> GSPGISGGGGGSAYSNTYQEFTNIDQAKAWGNAQYKKYGLSKSEKEAIVSYTKSASEINGKLRQNKGVINGFPSNLIKQVELLDKSFNKMKTPENIMLFRGDDPAYLGTEFQNTLLNSNGTINKTAFEKAKAKFLNKDRLEYGYISTSLMNVSQFAGRPIITKFKVAKGSKAG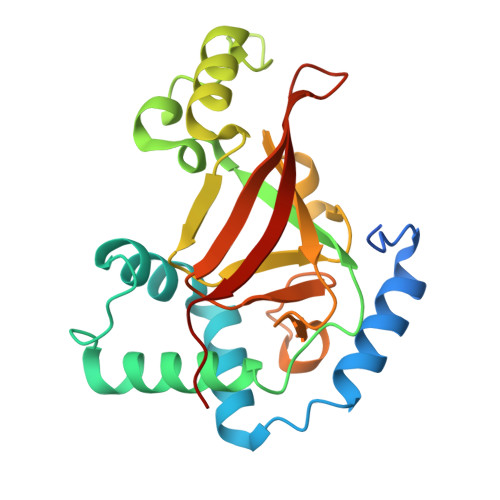YIDPISAFAGQLEMLLPRHSTYHIDDMRLSSDGKQIIITATMMGTAINPK>[4x]MVRFSRDMLQDGAKRMFKWLRKGEGLPNYLIMYDMDRNKEYKLVPKEYAGLYESRNIFWIKNGREPNYVTLTSVARNPLVMDYQNTNYTCCPTSLSLASQMLYHYKSESECAKALGTSKGSG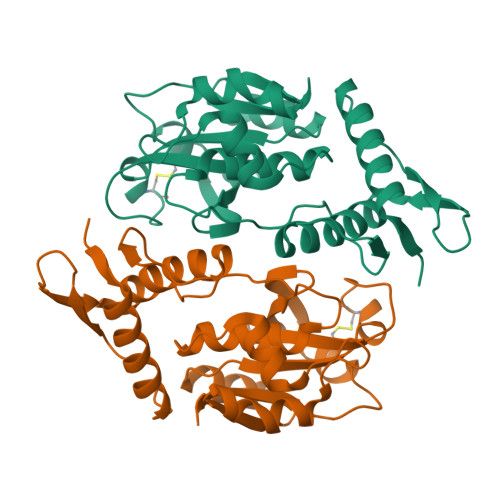TSPAQLIANAPKLGFKIIPIKRDSKEVKKYLKKGFPVICHWQVNQSRNCKGDYTGNFGHYGLIWDMTSTHYVVADPAKGVNRKYKFSCLDNANKGYRQNYYVVCPA> MGSSHHHHHHSQDPMVLLHKSTHIFPTDFASVSRAFFNRYPNPYSPHVLSIDTISRNVDQEGNLRTTRLLKKSG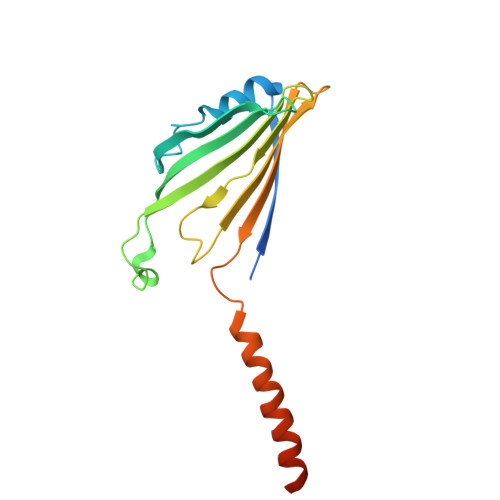KLPTWVKPFLRGITETWIIEVSVVNPANSTMKTYTRNLDHTGIMKVEEYTTYQFDSATSSTIADSRVKFSSGFNMGIKSKVEDWSRTKFDENVKKSRMGMAFVIQKLEEA> KDRPDFCELPADTGPCRVR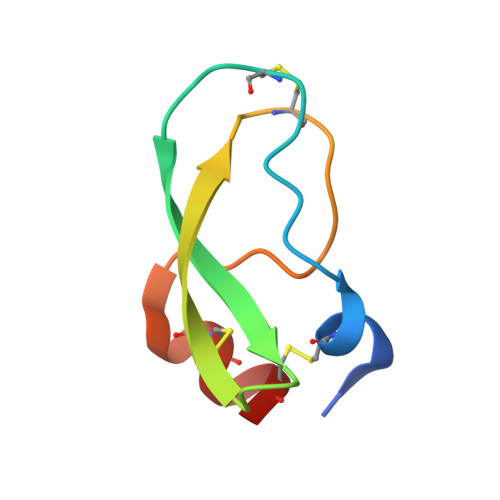FPSFYYNPDEKKCLEFIYGGCEGNANNFITKEECESTCAA> MAPGDIEDMIKAGIPGARVTIRDLAGDGDHYAAEVVAEA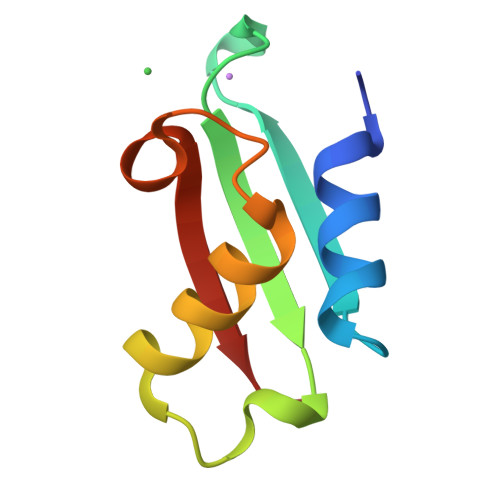FRGKTRVQQHQMVYNALKGNMGGILHALALQTSAPE Sarcosine oxidase from Bacillus sp. (SoxB) recognizes the cyclic imino acids l‐proline (l‐Pro), d‐proline (d‐Pro), and l‐thioproline (l‐Tpr) as minor substrates.

The Tyr254Ala and Tyr254Gly mutants exhibited enhanced reactivity toward cyclic imino acids by eliminating this spatial interference. Crystallographic analysis of the mutants revealed an enlarged active site, which facilitated reactions with five‐membered cyclic imino acids. These mutations disrupted the electron delocalization associated with l‐Tpr, thereby eliminating charge transfer and substrate inhibition.

>[2x]STHFDVIVVGAGSMGMAAGYQLAKQGVKTLLVDAFDPPHTNGSHHGDTRIIRHAYGEGREYVPLALRSQELWYELEKETHHKIFTKTGVLVFGPKGESAFVAETMEAAKEHSLTVDLLEGDEINKRWPGITVPENYNAIFEPNSGVLFSENCIRAYRELAEARGAKVLTHTRVEDFDISPDSVKIETANGSYTADKLIVSMGAWNSKLLSKLNLDIPLQPYRQVVGFFESDESKYSNDIDFPGFMVEVPNGIYGGFPSFGGCGLKLGYHTFGQKIDPDTINREFGVYPEDESNLRAFLEEYMPGANGELKRGAVCMYTKTLDEHFIIDLHPEHSNVVIAAGFSGHGFKFSSGVGEVLSQLALTGKTEHDISIFSINRPALKESLQKTTIGSHHHHHH> MSVIQNYNKALQQLEKYKPYEEALLQAEAPRLAEYQAYIDFEMKIGDPARIQLIFERALVENCLVPDLWIRYSQYLDRQLKVKDLVLSVHNRAIRNCPWTVALWSRYLLAMERHGVD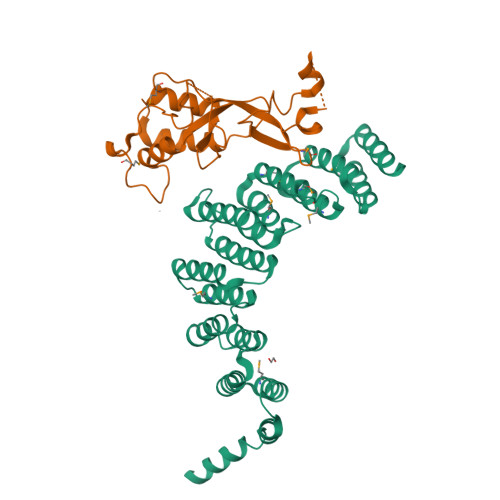HQVISVTFEKALNAGFIQATDYVEIWQAYLDYLRRRVDFKQDSSKELEELRAAFTRALEYLKQEVEERFNESGDPSCVIMQNWARIEARLCNNMQKARELWDSIMTRGNAKYANMWLEYYNLERAHGDTQHCRKALHRAVQCTSDYPEHVCEVLLTMERTEGSLEDWDIAVQKTETRLARVNE;> GMAEGGAADLDTQRSDIATLLKTSLRKGDTWYLVDSRWFKQWKKYVGFDSWDKYQMGDQNVYPGPIDNSGLLKDGDAQSLKEHLIDELDYILLPTEGWNKLVSWYTLMEGQEPIARKVVEQGMFVKHCKVEVYLTELKLCENGNMNNVVTRRFSKADTIDTIEKEIRKIFSIPDEKETRLWNKYMSNTFEPLNKPDSTIQDAGLYQGQVLVIEQKNEDGTWPRG> GMNNLYHLKVRCSSLHKIIGEPKSKADKEAGKLTDTAKSAVREMAKFDLFGYNAFEGNKYTQKGNELEEQAIKLSGVTRGLALKKNTERRENEFITGECDIYVPSRKLIIDTKCSWDIGSHPFFTDEAQEKAKKAGYDIQMQGYMWLWDCDQAQIDF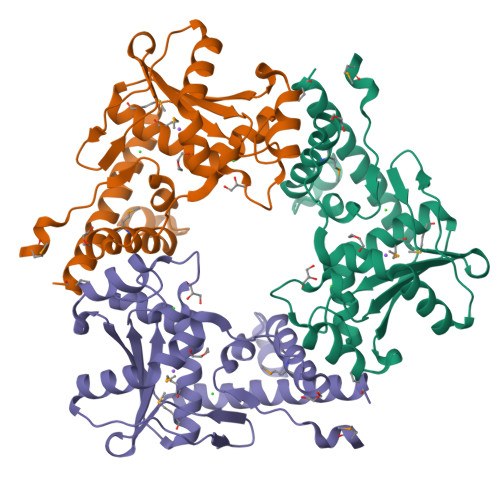VLFPTPLNLISAYDSDFKLIDLVEQIPQIRRITTVIIQRDNELIDKIKERVSAAQKYYDQLISEMS> GGAGGGGAAAUUCUAUCUGGUGAUAGACG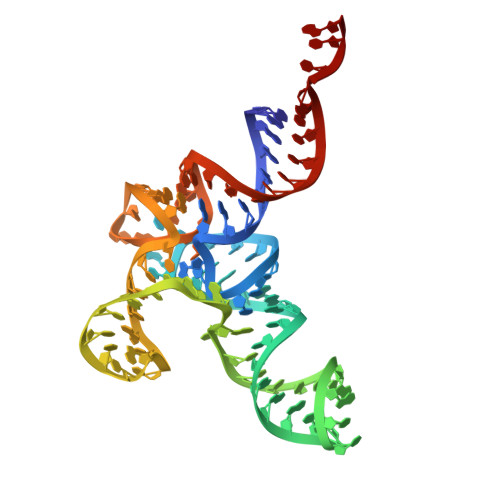GGAACUCUAAAUUCCUUGAAAUGCCUCGCCGCAUUGGGUUCGAUUCCCUUCCCCUCCGCCA>MAAGVAAWLPFARAAAIGWMPVASGPMPAPPRQERKRTQDALIVLNVSGTRFQTWQDTLERYPDTLLGSSERDFFYHPETQQYFFDRDPDIFR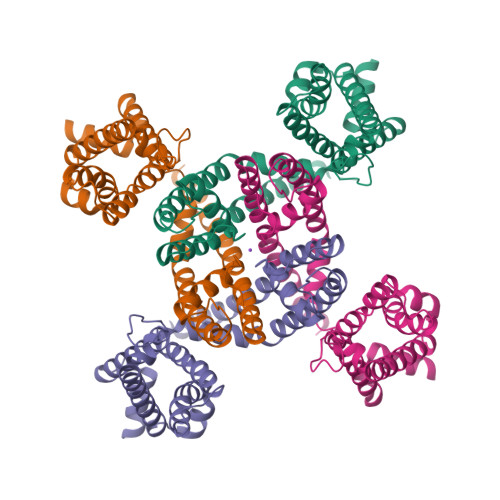HILNFYRTGKLHYPRHECISAYDEELAFFGLIPEIIGDCCYEEYKDRRRENAERLQDDADTDTAGESALPTMTARQRVWRAFENPHTSTMALVFYYVTGFFIAVSVIANVVETVPCGSSPGHIKELPCGERYAVAFFCLDTACVMIFTVEYLLRLAAAPSRYRFVRSVMSIIDVVAILPYYIGLVMTDNEDVSGAFVTLRVFRVFRIFKFSRHSQGLRILGYTLKSCASELGFLLFSLTMAIIIFATVMFYAEKGSSASKFTSIPAAFWYTIVTMTTLGYGDMVPKTIAGKIFGSICSLSGVLVIALPVPVIVSNFSRIYHQNQRADKRRAQKKARLARIRAAKSGSANAYMQSKRNGLLSNQLQSSEDEQAFVSKSGSSFETQHHHLLHCLEKTTNHEFVDEQVFEESCMEVATVNRPSSHSPSLSSQQG[4x]>MHHHHHHAGNSILLAAVSILSACQQSYFALQVGKARLKYKVTPPAVTGSPEFERVFRAQQNCVEFYPIFIITLWMAGWYFNQVFATCLGLVYIYGRH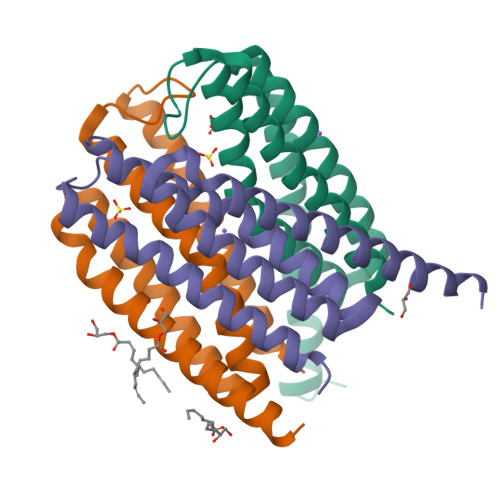LYFWGYSEAAKKRITGFRLSLGILALLTLLGALGIANSFLDEYLDLNIAKKLRRQF[6x]(3~{S},6~{S})-3-[(4-hydroxyphenyl)methyl]-6-[(3-methyl-4-oxidanyl-phenyl)methyl]piperazine-2,5-dione | C19 H20 N2 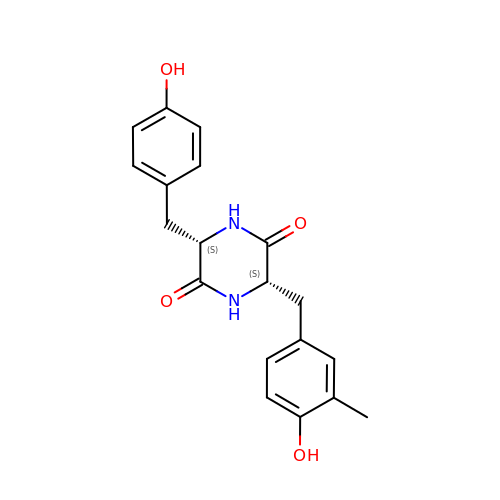O4 | YBIHVNADQSTKMY-HOTGVXAUSA-N> GPGSTEQAPPVRVLPERIHLHELDPNPPGPESDYRTRWEIPIGLRETDLTPAHCHMHTNPHLLIFGAAKSGKTTIAHAIARAICARNSPQQVRFMLA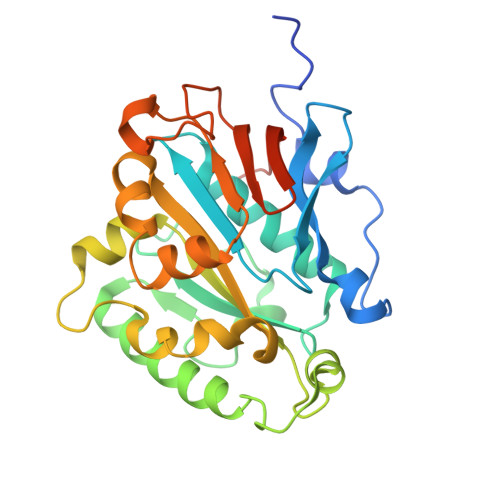DYRSGLLDAVPDTHLLGAGAINRNSASLDEAVQALAVNLKKRLPPTDLTTAQLRSRSWWSGFDVVLLVDDWHMIVGAAGGMPPMAPLAPLLPAAADIGLHIIVTCQMSQAYKATMDKFVGAAFGSGAPTMFLSGEKQEFPSSEFKVKRRPPGQAFLVSPDGKEVIQAPYIEPPEEVFAAPPSAG>[2x]AAESGELIGACEFMKDRLYFATLRNRPKSTINIHYFSIDEELVYENFYADFGPLNLAM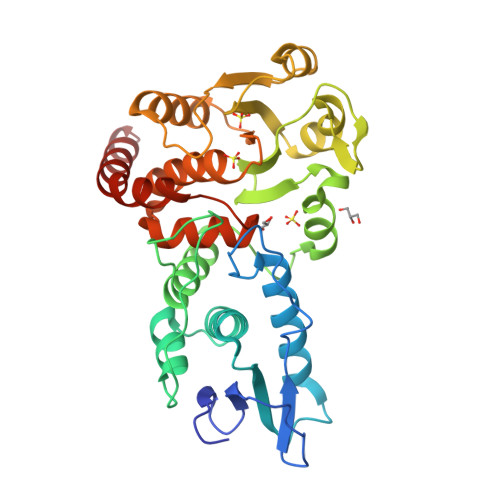VYRYCCKLNKKLKSYSLSRKKIVHYTSFDQRKRANAAFLIGAYAVIYLKKTPEEAYRALLSGSNPPYLPFRDASFGNCTYNLTVLDCLQGIRKGLQHGFFDFETFDAEEYEHYERVENGDFNWIVPGKFLAFSGPHPKSKIENGYPLHAPEAYFPYFKKNNVTTIVRLNKKIYEAKRFTDAGFEHYDLFFIDGSTPSDNIVRRFLNICENTEGAIAVHSKAGLGRTGTLIACYVMKHYRFTHAEIIAWIRICRPGSIIGPQQHFLKEKQASLWVQGDIFRSKLKNR>[2x]SMDMPVERILEAELAVEPKTESYGDMNMENSTNDPVTNICHAADKQLFTLVEWAKRIPHFSDLTLEDQVILLRAGWNELLIASFSHRSVSVQDGILLATGLHVHRSSAHSAGVGSIFDRVLTELVSKMKDMQMDKSELGCLRAIVLFNPDAKGLSNPSEVETLREKVYATLEAYTKQKYPEQPGRFAKLLL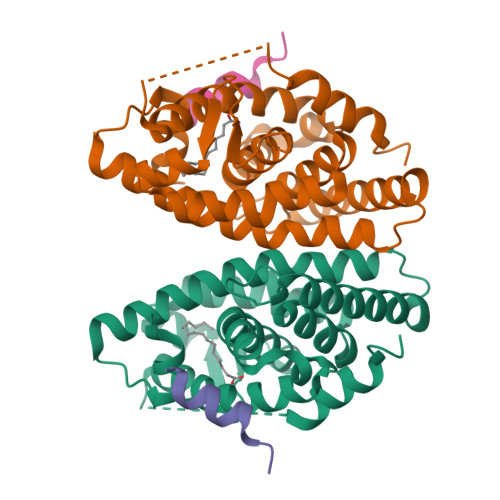RLPALRSIGLKCLEHLFFFKLIGDTPIDTFLMEMLETPLQIT;>KHKILHRLLQDSSY[2x]> GSHMNGEPDIAQLKGLSPSQRQAYAVQLKNRGNHFFTAKNFNEAIKYYQYAIELDPNEPVFYSNISACYISTGDLEKVIEFTTKALEIKPDHSKALLRRASANESLGNFTDAMFDLSVLSLNGDFDGASIEPMLERNLNKQAMKVLNENLSKDEGRGSQVLPSNTSLASFFGIFDSHLEVSSVNTSSNYDTAYALLSDALQRLYSATDEGYLVANDLLTKSTDMYHSLLSANTVDDPLRENAALALCYTGIFHFLKNNLLDAQVLLQESINLHPTPNSYIFLALTLADKENSQEFFKFFQKAVDLNPEYPPTYYHRGQMYFILQDYKNAKEDFQKAQSLNPENVYPYIQLACLLYKQGKFTESEAFFNETKLKFPTLPEVPTFFAEILTDRGDFDTAIKQYDIAKRLEEVQEKIHVGIGPLIGKATILARQSSQDPTQLDEEKFNAAIKLLTKACELDPRS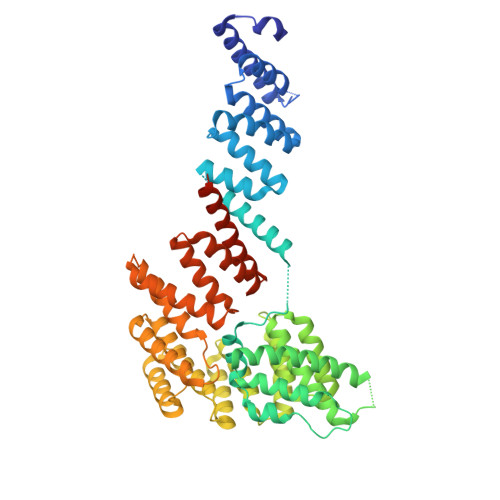EQAKIGLAQLKLQMEKIDEAIELFEDSAILARTMDEKLQATTFAEAAKIQKRLRADPIISAKMELTLARYRAKGML N-{1-[1,1-di(pyridin-2-yl)ethyl]-6-(5-{[(2-fluorophenyl)carbamoyl]amino}-1-methyl-6-oxo-1,6-dihydropyridin-3-yl)-1H-indol-4-yl}-2,2,2-trifluoroethane-1-sulfonamide 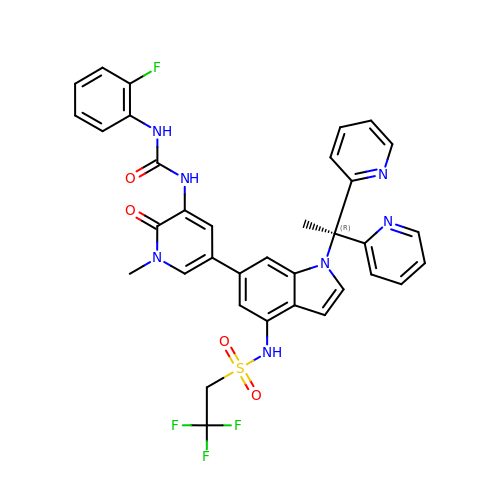| C35 H29 F4 N7 O4 S | RFUGSFUWHIKRES-UHFFFAOYSA-N>GCANNQTNASQPAEKNEKTEM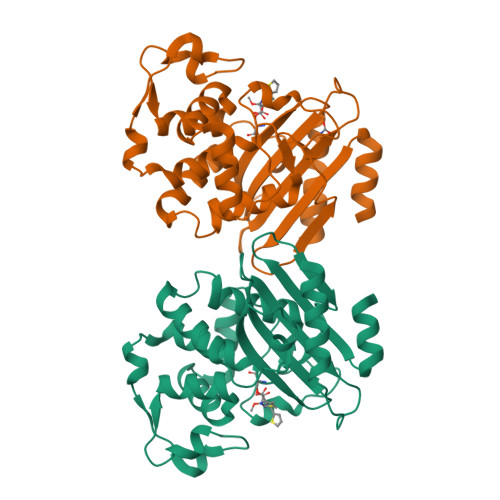KDDFAKLEEQFDAKLGIFALDTGTNRTVTYRPDERFAFASTIKALTVGVLLQQKSIEDLNQRITYTRDDLVNYNPITEKHVDTGMTLKELADASLRYSDNTAQNLILKQIGGPESLKKELRKIGDEVTNPERFEPELNEVNPGETQDTSTARALATSLQAFALEDKLPSEKRELLIDWMKRNTTGDALIRAGVPEGWEVADKTGAGSYGTRNDIAIIWPPKGDPVVLAVLSSRDKKDAKYDDKLIAEATKVVLKALNMNGK[2x]>MNIFSKDTDKGKHVSGIDRGKIVMYGLSTCVWCKKTKKLLTDLGVDFEYVFVDLLEEEEKSNAIKQVSRFNPSVSFPTTILNDEKAIVGFKEKQ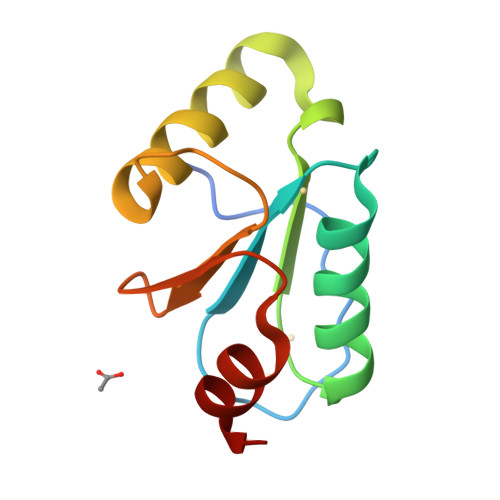IREALGF[4x]>[8x]MIGRLRGTLAEKQPPHLILDVNGVGY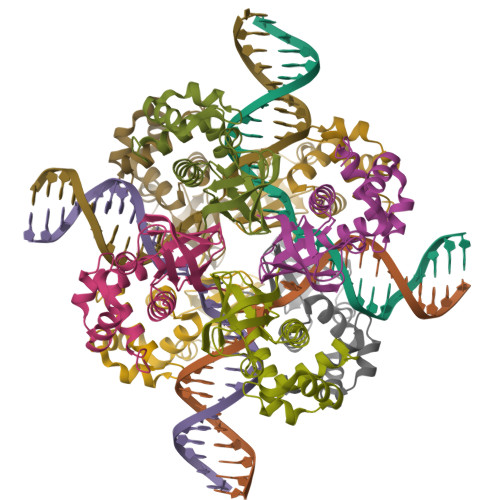EVEVPMTTLYRLPSVGEPVTLHTHLVVREDAHLLYGFAEKRERELFRELIRLNGVGPKLALALMSGLEVDELVRCVQAQDTSTLVKIPGVGKKTAERLLVELKDRFKAWEN> MDVIPLSLGLETMGGLVEKVIPRNTTIPVARAQDFTTFKDGQTAMSIHVMQGERELVQDCRSLARFALRGIPALPAGGAHIRVTFQVDADGLLSVTAMEKSTGVEASIQVKPSYGLTDSEIASMIKDSMSYAEQDVKARMLAEQKVEAARVLESLHGALAADAALLSAAERQVIDDAAAHLS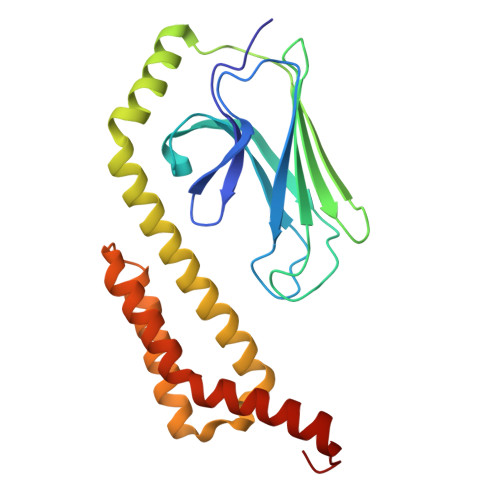EVAQGDDVDAIEQAIKNVDKQTQDFAARRMDQSVRRALKGHSVDE> EHQKEIQYEILQKTIPTFEPKESILKKLEDIKPEQAKKQTKLFRIFEPRQLPIYRANGEKELRNRWYWKLKKDTLPDGDYDVREYFLNLYDQVLTEMPDYLLLKDMAVENKNSRDAGKVVDSETASICDAIFQDEETEGAVRRFIAEMRQRVQADRNVVNYPSILHPIDYAFNEYFLQHQLVEPLNNDIIFNYIPERIRNDVNYILNMDRNLPSTARYIRPNLLQDRLNLHDNFESLWDTITTSNYILARSVVPDLKELVSTEAQIQKMSQDLQLEALTIQSETQFLTGINSQAANDCFKTLIAAMLSQRTMSLDFVTTNYMSLISGMWLLTVVPNDMFIRESLVACQLAIVNTIIYPAFGMQRMHYRNGDPQTPFQIAEQQIQNFQVANWLHFVNNNQFRQVVIDGVLNQVLNDNIRDGHVINQLMEALMQLSRQQFPTMPVDYKRSIQRGILLLSNRLGQLVDLTRLLAYNYETLMACVTMNMQHVQTLTTEKLQLTSVTSLCMLIGNATVIPSPQTLFHYYNVNVNFHSNYNERINDAVAIITAANRLNLYQKKMKAIVEDFLKRLHIFDVARVPDDQMYR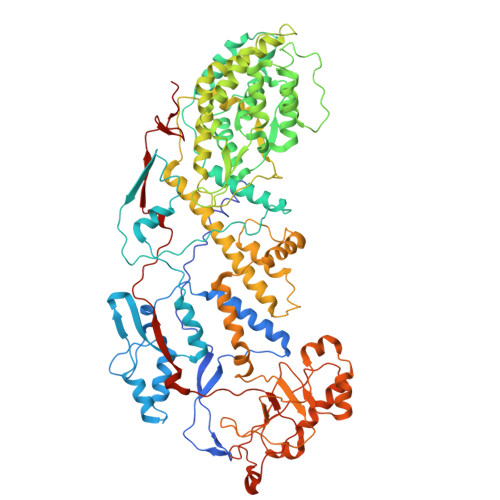LRDRLRLLPVEVRRLDIFNLILMNMDQIERASDKIAQGVIIAYRDMQLERDEMYGYVNIARNLDGFQQINLEELMRTGDYAQITNMLLNNQPVALVGALPFVTDSSVISLIAKLDATVFAQIVKLRKVDTLKPILYKINSDSNDFYLVANYDWVPTSTTKVYKQVPQQFDFRNSMHMLTSNLTFTVYSDLLAFVSADTVEPINAVAFDNMRIMNEL Some Gram-negative bacteria target their competitors by exploiting the type VI secretion system to extrude toxic effector proteins. To prevent self-harm, these bacteria also produce highly specific immunity proteins that neutralize these antagonistic effectors. The opportunistic pathogen Serratia marcescens has recently been shown to utilize T6-dependent secretion of two family 4 amidases, Ssp1 and Ssp2, to mediate antibacterial activity. In S. marcescens, the resistance-associated proteins Rap1a and Rap2a neutralize Ssp1 and Ssp2, respectively.

Rap2a, like Rap1a, is predicted to be localized in the periplasm and could only be produced in soluble recombinant form using the E. coli Rosetta-gami (DE3) strain. It is also a stable dimer in solution as shown by size-exclusion chromatography. The structure was determined at 1.9 Å resolution with four molecules, arranged as two dimers, in the asymmetric unit. These four molecules, sub­units A–B and C–D, are similar overall, with r.m.s.d.s between superimposed Cα atoms ranging from 0.6 Å (subunits A and B, residues Thr27–Gln123) to 0.7 Å (subunits C, residues 27–127, and D, residues 27–126). Minor deviations from NCS are observed in a five-residue loop between α2 and α3 (Gly67–Leu71) and indicate some conformational freedom in this part of the molecule. The ASA of a Rap2a subunit averages at approximately 6110 Å2; the range is from 6140 Å2 for subunit C to 6090 Å2 for subunit D. Dimer formation occludes an area that is approximately 20% of the ASA, which is indicative of a stable association. A disulfide bond between Cys42 and Cys102 links α1 to α4 and interactions of other side-chain groups on these elements of secondary structure help to create the helical bundle fold and in particular to align α2. Together, α1, α2, the α2–α3 loop and α4 form the dimer interface, giving rise to a twofold NCS axis, and a combination of hydrogen-bonding, salt-bridge and van der Waals interactions serve to stabilize the association. The side chains of Leu39, Ile43, Tyr47, Val52, Met99 and Ile103 are involved in van der Waals interactions with the partner subunit to stabilize the dimer.

>GHMKETYTPEEYLKNYALSVCIAEGYSAKEVKNDAAAAARGYTEFGDYSLEAHTAVRALAKEFLAKPYDSMSGEPMTMAKCIDLVHSQELQAIIKKYQGKDDN[4x]>ARSEKRVPMTRLRKRVAERLLEAKNSTAMLTTFNEVNMKPIMDLRKQYGEAFEKRHGIRLGFMSFYVKAVVEALKRYPEVNASIDGDDVVYHNYFDVSMAVSTPRGLVTPVLRDVDTLGMADIEKKIKELAVKGRDGKLTVEDLTGGNFTITNGGVFGSLMSTPIINPPQSAILGMHAIKDRPMAVNGQVEILPMMYLALSYDHRLIDGRESVGFLVTIKELLEDPTRLLLDV[24x]

DLST is an octahedral subunit of the E2 component of the ɑ-ketoglutarate dehydrogenase complex (KGDHC), which plays a pivotal role in the tricarboxylic acid (TCA) cycle, converting ɑ-ketoglutarate to succinyl-Coenzyme A and reducing nicotinamide adenine dinucleotide (Sheu and Blass, 1999, Knapp et al., 2000, Andi et al., 2019). The complex has three structured domains linked together by a chain of unstructured residues, with the C-terminal domain being the catalytic domain where multiple DLST subunits interact to form the full 24-subunit assembly. Notably, DLST has previously been observed as a contaminant protein in samples purified from E. coli expression systems (Bolanos-Garcia and Davies, 1760 (2006), Andi et al., 2019).

During the assembly and purification of a novel two-component protein nanoparticle with designed octahedral symmetry (to be detailed in an upcoming publication), we discovered that a significant portion of the purified sample consisted of a smaller, unidentified protein complex, which also exhibited octahedral symmetry, as revealed by ns-EM. However, the predominant species observed by ns-EM was a smaller, cube-like particle lacking the distinctive spiked features of our intended design. To identify the unknown nanoparticle in the absence of a corresponding amino acid sequence or prior structural information, we turned to the automated model-building software ModelAngelo. Running ModelAngelo in this manner on our 2.51 Å Cryo-EM map generated 92 all-atom sequence fragments of varying lengths, along with secondary structure predictions that were in strong agreement with the density of the unknown nanoparticle. Following the Protein BLAST result, a pairwise sequence alignment using EMBOSS Needle between the Uniprot sequence A0A140NDX4 of DLST from E. coli BL21 (DE3) and the ModelAngelo-derived consensus sequence was performed. This pairwise sequence alignment excluded the first 170 residues of DLST that were unresolved in our Cryo-EM map. Similarly, AlphaFold 3 (AF3) predictions using the catalytic domain of the A0A140NDX4 UniProt sequence also showed high agreement with our Cryo-EM map (UniProt, (n.d.), Abramson et al., 2024). To generate our final DLST catalytic domain model, the DLST sequence derived from E. coli BL21(DE3) was used as the input for another round of automated model building, this time utilizing the sequence-guided feature in ModelAngelo with the UniProt sequence for DLST (UniProt, (n.d.)). 100 mM glycine and 100 mM arginine were added to all purification buffers to mitigate potential off-target interactions between our nanoparticle and DLST, which resulted in the near-complete removal of DLST in all ns-EM micrographs of these purified samples.3,5-dimethylpyrazin-2(1H)-one 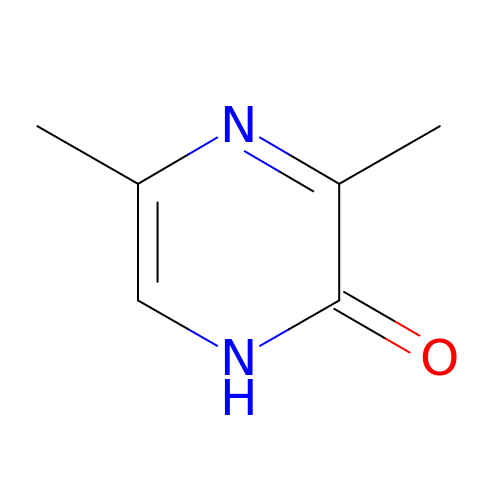| C6 H8 N2 O | AJYKJVCIKQEVCF-UHFFFAOYSA-N> MPGMELSPELLRKLETLAKIRLSPEEEALLLQDLKRILDFVDALPRV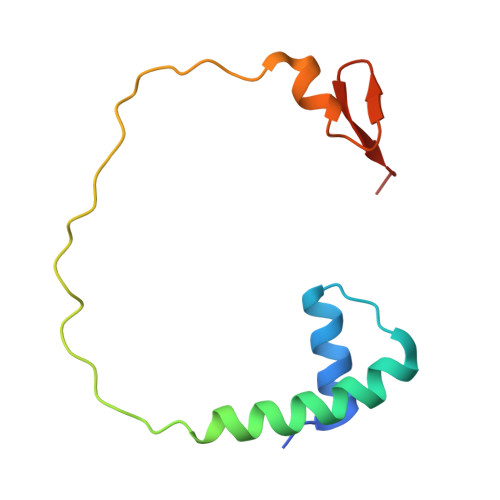EEGGAEEALGRLREDEPRPSLPQAEALALAPEAEDGFFRVPPVLE> MSEENLRPAYDDQVNEDVYKRGAQSKLTKARKADFDDEKDKKKDNDKHIDKRPKSGPRLDENGNPLPKEPRLPKRKVAVMVGYCGTGYHGMQYNPPNPTIESALFKAFVEAGAISKDNSNDLKKNGFMRAARTDKGVHAGGNLISLKMIIEDPDIKQKINEKLPEGIRVWDIERVNKAFDCRKMCSSRWYEYLLPTYSLIGPKPGSILYRDIEESKTELPGVLDEDLESKEFWEEFKKDANEKFSTEEIEAILAYVPPARDEFDINEELYQKVKKYKQLENAHRRRYRISAAKLAKFRASTSQYLGAHNFHNFTLGKDFKEPSAIRFMKDIKVSDPFVIGDAQTEWISIKIHGQSFMLHQIRKMV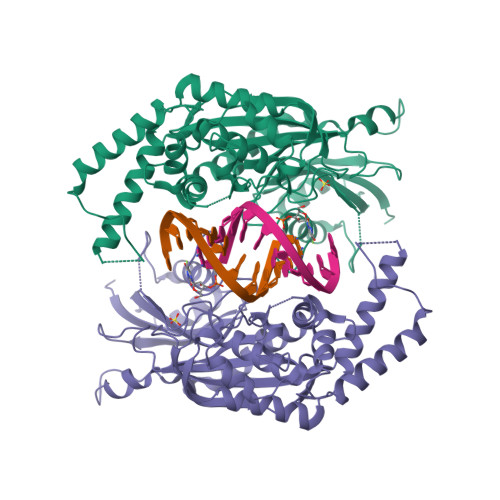SMATLITRCGCPVERISQAYGQQKINIPKAPALGLLLEAPVFEGYNKRLEQFGYKAIDFSKYQDEVDKFKMKHIYDKIYKEEVDENVFNAFFSYIDSFNKVTGAQGEETADKSGPAVQKSIFEFLTAKGIPGLTDAPESNKKIKQRKRMEEEEAASKKAEISSTTQSNEPEVQPEAAAN>[6x]MDQTYSLESFLNHVQKRDPNQTEFAQAVREVMTTLWPFLEQNPKYRQMSLLERLVEPERVIQFRVVWVDDRNQIQVNRAWRVQFSSAIGPYKGGMRFHPSVNLSILKFLGFEQTFKNALTTLPMGGGKGGSDFDPKGKSEGEVMRFCQALMTELYRHLGADTDV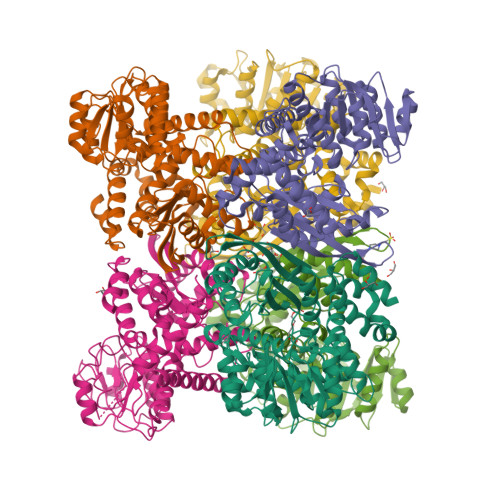PAGDIGVGGREVGFMAGMMKKLSNNTACVFTGKGLSFGGSLIRPEATGYGLVYFTEAMLKRHGMGFEGMRVSVSGSGNVAQYAIEKAMEFGARVITASDSSGTVVDESGFTKEKLARLIEIKASRDGRVADYAKEFGLVYLEGQQPWSLPVDIALPCATQNELDVDAAHQLIANGVKAVAEGANMPTTIEATELFQQAGVLFAPGKAANAGGVATSGLEMAQNAARLGWKAEKVDARLHHIMLDIHHACVEHGGEGEQTNYVQGANIAGFVKVADAMLAQGVI N-oxidanyl-2-[4-(4-sulfamoylphenyl)phenyl]ethanamide | C14 H14 N2 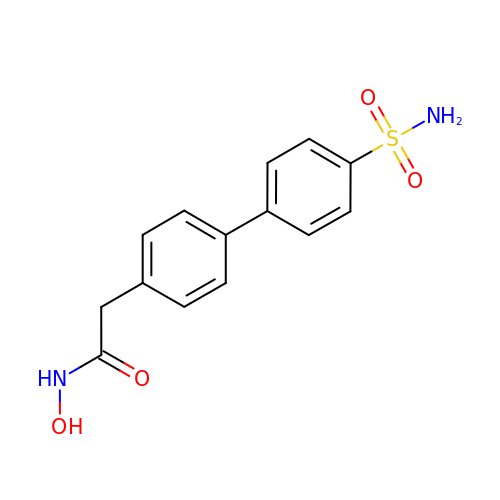O4 S | PHUYCWVFVRSGMR-UHFFFAOYSA-N>MQLTTLFNDDSAVSPVIGVILMVAITVILAAVI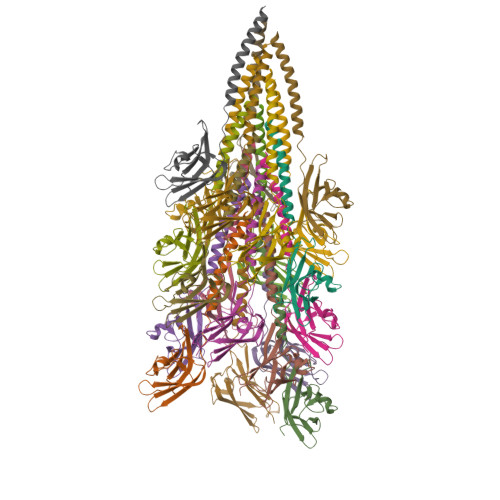GTFVLGLGDQVSETSPQASFDFDYTNTSGNLTITHESGTSIDADSVSISGPVGDDGKTWADIDGSATEITAGSSITVTANGSSFDSGETVRVIWTSDSGSSSSTLQSWTYNG[20x]>[6x]RGSHMNIKQFDILYIDLNPTRGREKHNVRPCLVINNQMSIDGTNFVWVLPITTRGLRYPTDIQLKTKKGLVSGVIDTVQIRALDLKARQYN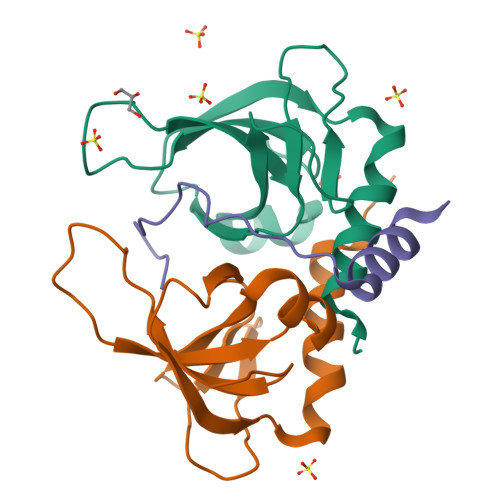YKDELQDNLKNDILKAIKTYLKPTL;>KSIEDRIKNFFQSGGKYTELEVDWEERVGREI[3x]> SWESHKSGGET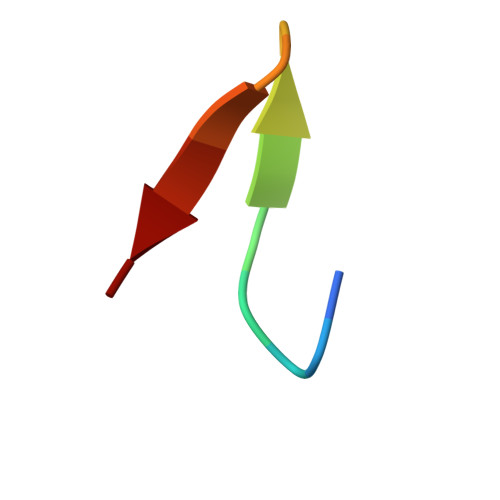RL> GPISPIETVPVKLKPGMDGPKVKQWPLTEEKIKALVEICTEMEKEGKISKIGPENPYNTPVFAIKKKDGTKWRKLVDFRELNKKTQDFWEVQLGIPHPAGLKKKKSVTVLDVGDAYFSVPLDEDFRKYT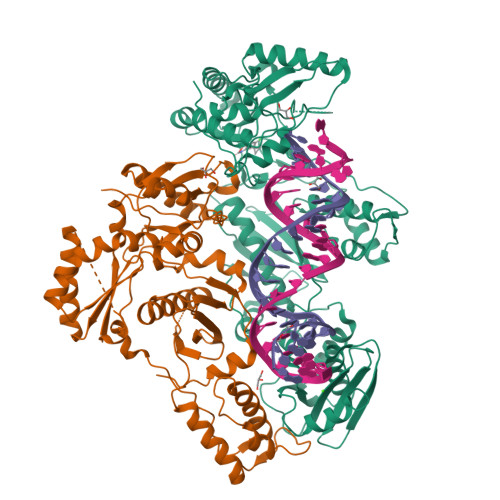AFTIPSINNETPGIRYQYNVLPQGWKGSPAIFQSSMTKILEPFRKQNPDIVIYQYMDDLYVGSDLEIGQHRTKIEELRQHLLRWGLTTPDKKHQKEPPFLWMGYELHPDKWTVQPIVLPEKDSWTVNDIQKLVGKLNWASQIYPGIKVRQLCKLLRGTKALTEVIPLTEEAELELAENREILKEPVHGVYYDPSKDLIAEIQKQGQGQWTYQIYQEPFKNLKTGKYARMRGAHTNDVKQLTEAVQKITTESIVIWGKTPKFKLPIQKETWETWWTEYWQATWVPEWEFVNTPPLVKLWYQLEKEPIVGAETFYVDGAASRETKLGKAGYVTNKGRQKVVTLTDTTNQKTELQAIHLALQDSGLEVNIVTDSQYALGIIQAQPDQSESELVNQIIEQLIKKEKVYLAWVPAHKGIGGNEQVDKLVSAGIR;> GPISPIETVPVKLKPGMDGPKVKQWPLTEEKIKALVEICTEMEKEGKISKIGPENPYNTPVFAIKKKDGTKWRKLVDFRELNKKTQDFWEVQLGIPHPAGLKKKKSVTVLDVGDAYFSVPLDEDFRKYTAFTIPSINNETPGIRYQYNVLPQGWKGSPAIFQSSMTKILEPFRKQNPDIVIYQYMDDLYVGSDLEIGQHRTKIEELRQHLLRWGLTTPDKKHQKEPPFLWMGYELHPDKWTVQPIVLPEKDSWTVNDIQKLVGKLNWASQIYPGIKVRQLCKLLRGTKALTEVIPLTEEAELELAENREILKEPVHGVYYDPSKDLIAEIQKQGQGQWTYQIYQEPFKNLKTGKYARMRGAHTNDVKQLTEAVQKITTESIVIWGKTPKFKLPIQKETWETWWTEYWQATWVPEWEFVNTPPLVKLWYQLEKEPIVGAETF> MAPFRQDSILIIYPRSQTTLVQFGLNEETFTVPELEIPTQIYRTTRQDGSYTYHSTNKDNKAELIKPIQNGEIIDISAFTQFLRLIFVSILSDRANKNQDAFEAELSNIPLLLITHHSWSQSDLEIITQYVFESLEINNLIQLPASLAATYSMISLQNCCIIDVGTHHTDIIPIVDYAQLDHLVSSIPMGGQSINDSLKKLLPQWDDDQIESLKKSPIFEVLSDDAKKLSSFDFGNENEDEDEGTLKNSDLEFNTFWDEKGNEIKVGKQRFQGCNNLIKNISNRVGLTLDNIDDINKAKAVWENIIIVGGTTSISGFKEALLGQLLKDHLIIEPEEEKSKREEEAKSVLPAATKKKSKFMTNSTAFVPTIEYVQCPTVIKLAKYPD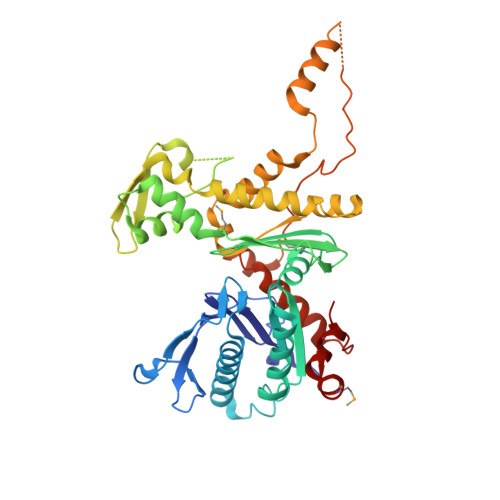YFPEWKKSGYSEIIFLGAQIVSKQIFTHPKDTFYITREKYNMKGPAALWDVQF> MPAAPLDVKCLEANKDYIIISWKQPAVDGGSPILGYFIDKCEVGTDSWSQCNDTPVKFARFPVTGLIEGRSYIFRVRAVNKMGIGFPSRVSEPVAALDPAEKARLKSRPSAPWTGQIIVTEEEPSEGIVPGPPTDLSVTEATRSYVVLSWKPPGQRGHEGIMYFVEK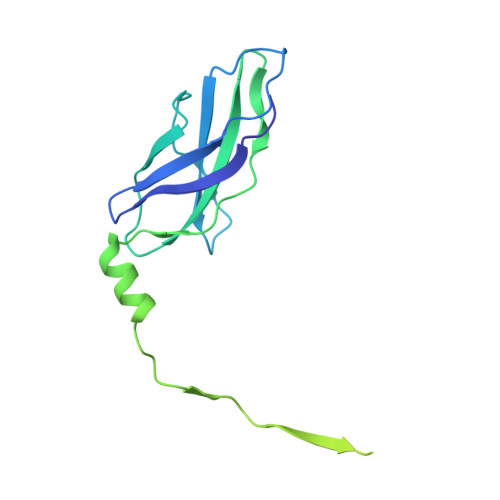CEAGTENWQRVNTELPVKSPRFALFDLAEGKSYCFRVRCSNSAGVGEPSEATEVTVVGDKLDIP> MDIVDGDQCESNPCLNGGSC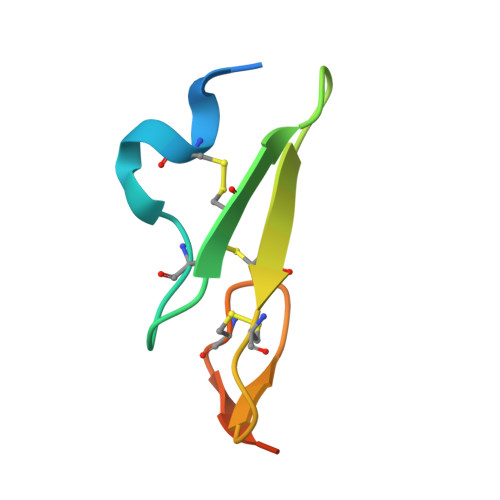KDDINSYECWCPFGFEGKNCELLEHHHHHH> 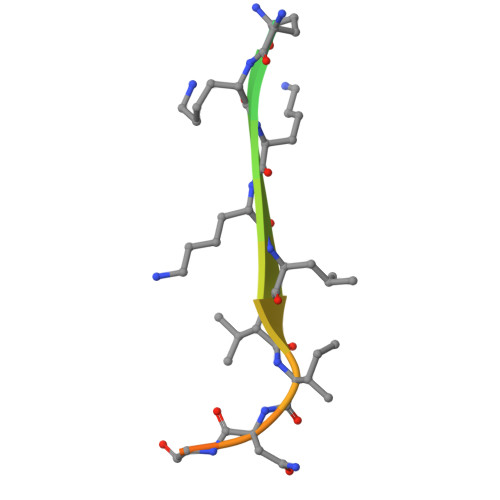SRRRCGQKKKLVINGGNGTV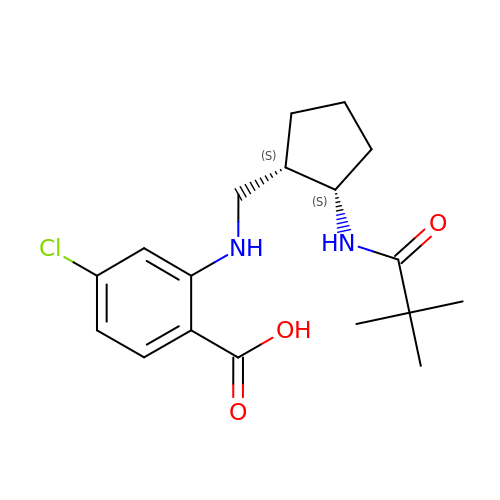4-chloro-2-[({(1S,2S)-2-[(2,2-dimethylpropanoyl)amino]cyclopentyl}methyl)amino]benzoic acid | C18 H25 Cl N2 O3 | KOHMGERIGIVBEC-FZMZJTMJSA-N>IVGGYECKAYSQPHQVSLNSGYHFCGGSLVNENWVVSAAHCYKSRVAVRLGEHNIKVTEGSEQFISSSRVIRHPNYSSYNIDNDIMLIKLSKPATLNTYVQPVALPSSCAPAGTMCTVSGWGNTMSSTADGDKLQCLNIPILSYSDCNNS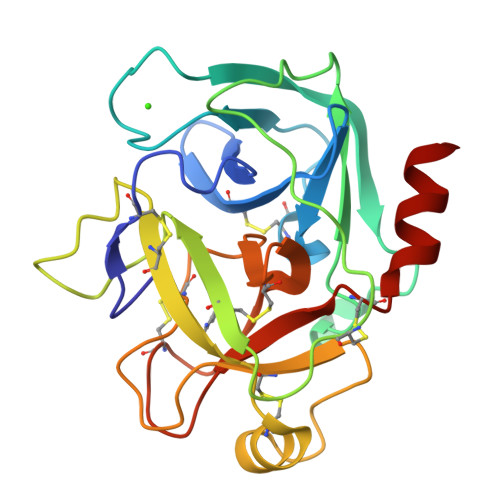YPGMITNAMFCAGYLEGGKDSCQGDSGGPVVCNGELQGVVSWGYGCAEPGNPGVYAKVCIFNDWLTSTMATY[2x]>SLTRIDHIGIACHDLDATVEFYRATYGFEVFHTEVNEEQGVREAMLKINDTSDGGASY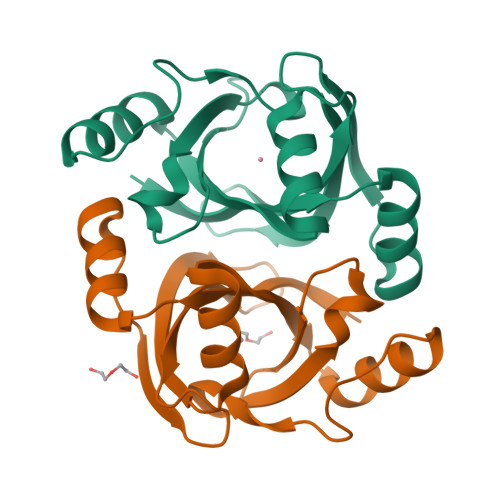LQLLEPTREDSAVGKWLAKNGEGVHHIAFGTADVDADAADIRDKGVRVLYDEPRRGSMGSRITFLHPKDCHGVLTELVTSAAVESPEH[2x]>SYYHHHHHHLESTSLYKKAGAFAAKDVVVAVGSNFTTLDPYDANDTLSQAVAKSFYQGLFGLDKEMKLKNVLAESYTVSDDGITYTVKLREGIKFQDGTDFNAAAVKANLDRASDPANHLKRHNLYKNIAKTEAIDPTTVKITLKQPFSAFINILAHPATAMISPAALEKYGKEIGFYPVGTGPYELDTWNQTDFVKVKKFAGYWQPGLPKLDSITWRPVADNNTRAAMLQTGEAQFAFPIP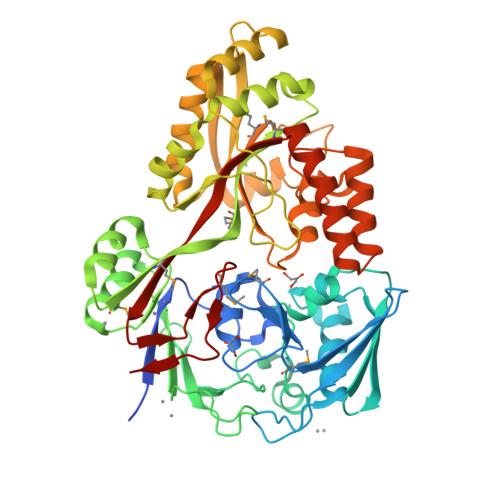YEQATLLEKNKNIELMASPSIMQRYISMNVTQKPFDNPKVREALNYAINRPALVKVAFAGYATPATGVVPPSIAYAQSYKPWPYDPVKARELLKEAGYPNGFSTTLWSSHNHSTAQKVLQFTQQQLAQVGIKAQVTAMDAGQRAAEVEGKGQKESGVRMFYTGWSASTGEADWALSPLFASQNWPPTLFNTAFYSNKQVDDFLAQALKTNDPAEKTRLYKAAQDIIWQESPWIPLVVEKLVSAHSKNLTGFWIMPDTGFSFEDADLQ[2x]>MAFELPKLPYAFDALEPHFDKETMEIHHDRHHNTYVTKLNAAVEGTDLESKSIEEIVANLDSVPANIQTAVRNNGGGHLNHSLFWELLSPNSEEKGTVVEKIKEQWGSLEEFKKEFADKAAARFGSGWAWLVVNNGQLEIVTTPNQDNPLTEGKTPILLFDVWEHAYYLKYQNKRPDYIGAF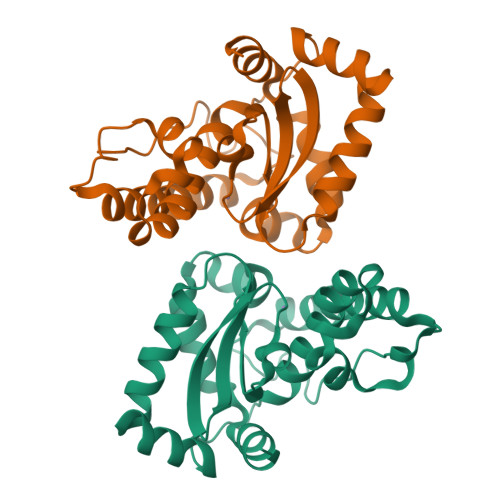WNVVNWEKVDELYNATK[2x]> GSHMSNKEYRPTLAQLRTFVTIAECKHFGTAATKLSISQPSLSQALVALETGLGVQLIERSTRKVIVTPAGEKLLPFAKSTLDAAESFLSHAKGANGSLTGPLTVGIIPTAAPYILPSMLSIVDEEYPDLEPHIVEDQTKHLLALLRDGAIDVAMMALPSEAPGMKEIPLYDEDFIVVTASDHPFAGRQDLELSALEDLDLLLLDDGHCLHDQIVDLCRRGNINPISSTTAVTRASSLTTVMQLVVAGLGSTLVPISAIPWECTRPGLATANFNSDVTANRRIGLVYRSSSSRAEEFEQFALILQRAFQEAVALAASTGITLK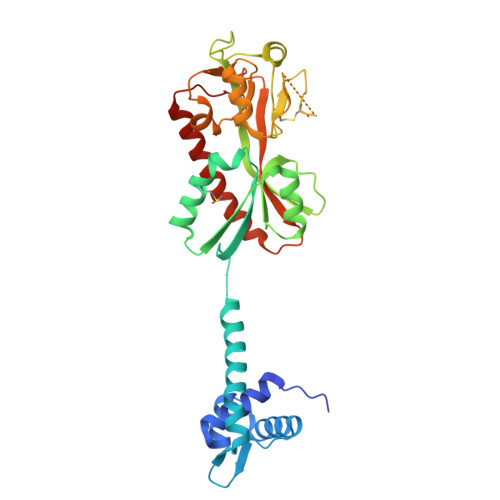QNVA In eukaryotes, integration of sterols into the vacuolar/lysosomal membrane is critically dependent on the Niemann–Pick type C (NPC) system. The system consists of an integral membrane protein, called NCR1 in yeast, and NPC2, a luminal soluble protein that transfers sterols to the N-terminal domain (NTD) of NCR1 before membrane integration. NCR1 and hNPC1 share the same structural fold: an N-terminal domain (NTD), a middle-luminal domain, and a C-terminal domain found on the luminal side of the vacuolar/lysosomal membrane. The current transport model for the NPC system postulates that NPC2 binds sterols in the lumen and loads them into the NTD, which transfers the sterol to a tunnel that is formed by the middle-luminal domain and C-terminal domain of hNPC1 and NCR1, respectively.

To study the substrate scope of NCR1, the NTD (residues 1–249 of NCR1) was purified and crystallized with either ergosterol or cholesterol: ergosterol-bound structure at 2.4 Å (Rfree 26%) and cholesterol-bound structure at 2.6 Å (Rfree 26%). Besides the sterol, the two structures show minimal differences between them (root mean square deviation of C-alpha atoms, RMSDCα, of 0.39 Å). Ergosterol and cholesterol are highly similar in their chemical structure, but the quality of the electron density maps allows for clear discernment between the two in the NTD binding pocket. In particular, the double bond between C22 and C23 of ergosterol results in a more rigid iso-octyl chain, evident as density that is continuous with the ring system. The hydroxyl group of ergosterol is coordinated by Q80, 3.0 Å away. The interior of the substrate binding pocket is lined with hydrophobic residues, except for Q80, N87, T113, and S196—with Q80 coordinating the hydroxyl group of the sterol. F109 and F112 are positioned underneath the ligand, allowing for pi-stacking with the sterol ring system. When comparing the position of ergosterol in the crystal structure of the NTD at pH 6 of this study to that of the full-length NCR1 solved by cryo-EM, the sterol position differs. The ergosterol is bound ∼4.5 Å deeper in the binding pocket of the crystal structure compared with the cryo-EM structures. One explanation for this is that the crystal structure of the NTD represents a post-loading state, whereas the cryo-EM structures show the sterol approaching the transfer state.

>[4x]MNVLWIIALVGQLMRLVQGTATCAMYGNCGKKSVFGNELPCPVPRSFEPPVLSDETSKLLVEVCGEEWKEVRYACCTKDQVVALRDNLQKAQPLISSCPACLKNFNNLFCHFTCAADQGRFVNITKVEKSKEDKDIVAELDVFMNSSWASEFYDSCKNIKFSATNGYAMDLIGGGAKNYSQFLKFLGDAKPMLGGSPFQINYKYDLANEEKEWQEFNDEVYACDDAQYKCACSDCQESCPHLKPLVPR>WSHPQFEKGAETAVPNSSSYGSRIEREQHHLIESIEKSTQYMAKRRIGALISVARDTGMDDYIETGIPLNAKISSQLLINIFIPNTPLHDGAVIIKGNEIASAASYLPLSDSPFLSKELGTRHRAALGISEVTDSITIVVSEETGGISLTKGGELFRDVSEEELHKILLKELVTVTAKKPSIF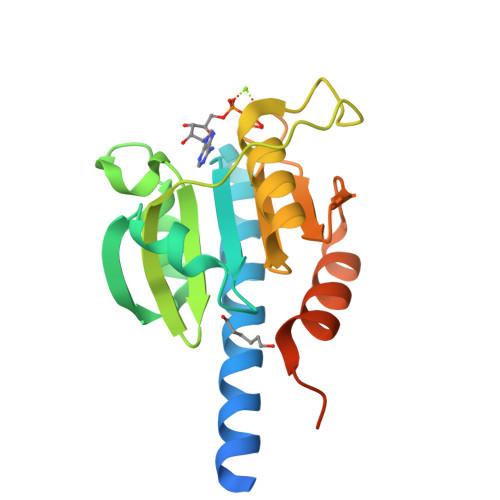SKWKGGKSE[4x]>GSHMANLDRTDDLVYLNVMELVRAVLELKNELSQLPPEGYVVVVKNVGLTLRKLIGSVDDLLPSLPSSSRTEIEGTQKLLNKDLAELINKMRLAQQNAVTSLSEECKRQMLTASHTLAVDAKNLLDAVDQAKVLANLAH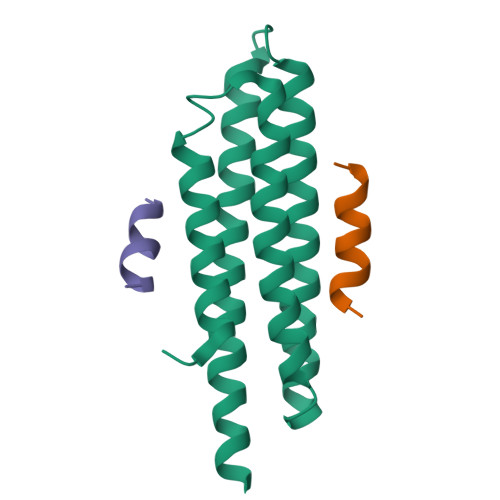[4x];>SATRELDELMASLSDFK[6x]> GMKRAVVVFSGGQDSTTCLIQALQDYDDVHCITFDYGQR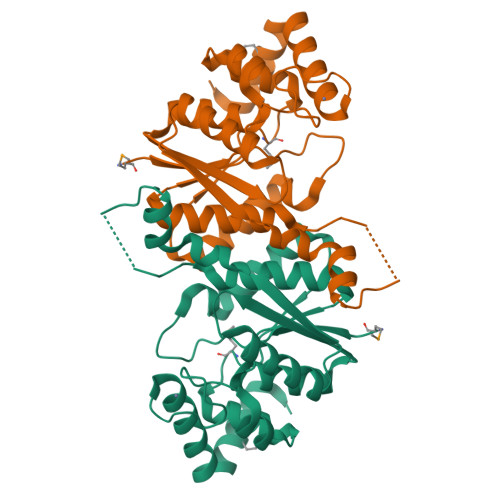HRAEIEVAQELSQKLGAAAHKVLDVGLLNELATSSLTRDSIPVPDYDANAQGIPNTFVPGRNILFLTLASIYAYQVGAEAVITGVCETDFSGYPDCRDEFVKALNQAIVLGIARDIRFETPLMWLNKAETWALADYYQQLDTVRYHTLTCYNGIKGDGCGQCAACHLRANGLAQYQKDAATVMASLKQKVGLR> MSHQERLQSKSLHLSPQEQSASYQDRRQSWRRASMKETNRRKSLHPIHQGITELSRSISVDLAESKRLGCLLLSSFQFSIQKLEPFLRDTKGFSLESFRAKASSLSEELKHFADGLETDGTLQKCFEDSNGKASDFSLEASVAEMKEYITKFSLERQTWDQLLLHYQQEAKEILSRGSTEAKITEVKVEPMTYLGSSQNEVLNTKPDYQKILQNQSKVFDCMELVMDELQGSVKQLQAFMDESTQCFQKVSVQLGKRSMQQLDPSPARKLLKLQLQNPPAIHGSGSGSCQHHHHH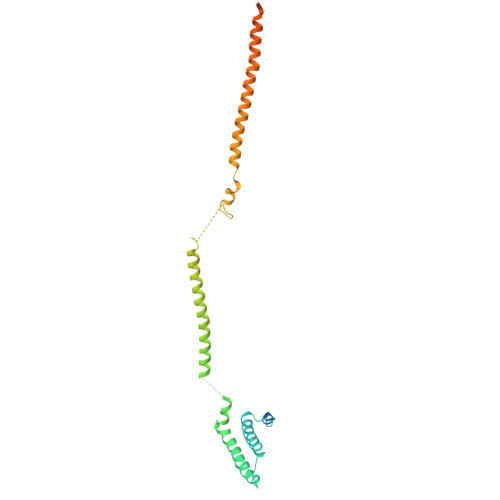H> MSKVMKPSNGKGSRKSSKAATPDTKNFFHAKKKDPVNQDKANNASQITPTVPHSHPSDMVIPDHLAELIPELYSFQQLVDSEKRLDHFIHLRNLHMKRMVAQWERSKLSQEFLYPHLNFPNVKFLRIFISNVSENQPWQMDTNNEADLMALENATWTMRIEGRLLDNVQANDPAREKFSSFIESIVVDFKNKENDNVPSTKFNAAPEENATEGPSDKKLNLNLPLQFSLPNGDNSTTTNTDQNNATMGEETAKKDMSSTTPKLESVKWQYDPNNPVDFDGLDIKRVGSENVECTISILRKSSPEEPFMSYSPQLTAIIGLKSGTSHDAIFSIYKYIHLNELLTNDESAFENLMGNRNNHNSNTSTSKMLDAASSQVSIVKLDTQLITLLPSSLKESSPDTMKLTDLLS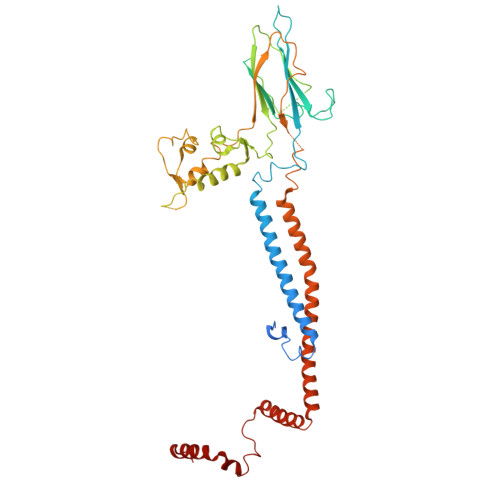LINSTHLLPLQPIEIDYTVRVDKASTYGELVLDIEVPDVNALKFNNTQRESQIGAAELNENARELEQIKPKIALQDKEITSVLSNLHESNKRYRFFKKISEDPVKALNECIASTSNALKVLSGDEGYNEDMVRRANFYKENEAMLRENIEVILSNGRM> DFDFLKNLSLEELQMRLKALDPMMER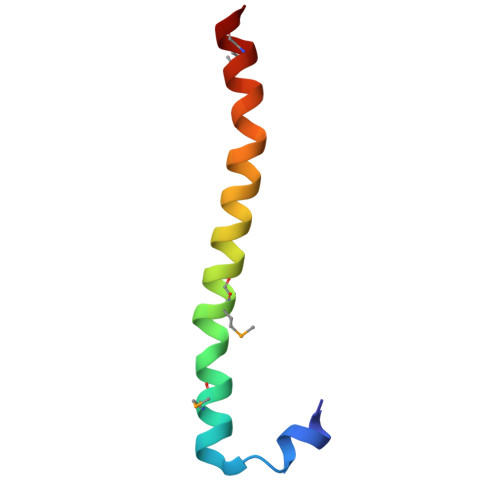EIEELRQRYTAKRQPILDAMDAK> MIIIRYLVRETLKSQLAILFILLLIFFCQKLVRILGAAVDGDIPANLVLSLLGLGVPEMAQLILPLSLFLGLLMTLGKLYTESEITVMHACGLSKAVLVKAAMILAVFTAIVAAVNVMWAGPWSSRHQDEVLAEAKANPGMAALAQGQFQQATNGSSVLFIESVDGSDFKDVFLAQIRPKGNARPSVVVADSGHLTQLRDGSQVVTLNQGTRFEGTALLRDFRITDFQDYQAIIGHQAVALDPNDTDQMDMRTLWNTDTDRARAELNWRITLVVTVFMMALMVVPLS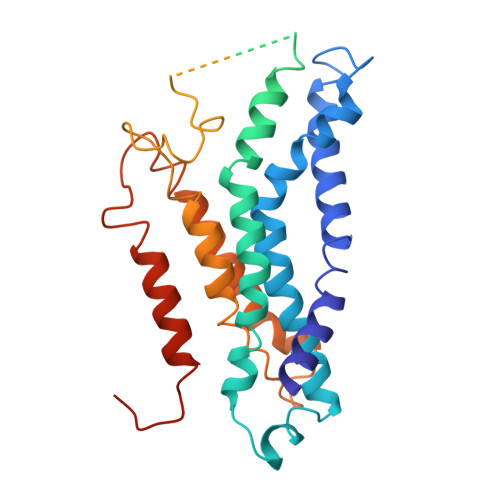VVNPRQGRVLSMLPAMLLYLLFFLIQTSLKSNGGKGKLDPTLWMWTVNLIYLALAIVLNLWDTVPVRRLRASFSRKGAV>[2x]GALARPCDCDVGGALDPQCDEATGQCRCRPHMIGRRCEQVQPGYFRPFLDHLTWEAEGAHGQVLEVVERLVTNRETPSWTGVGFVRLREGQEVEFLVTSLPRAMDYDLLLRWEPQVPEQWAELELVVQRPGPVSAHSPCGHVLPRDDRIQGMLHPNTRVLVFPRPVCLEPGLSYKLKLKLTGTGGRAHPETPYSGSGILIDSLVLQPHVLMLEMFSGGDAAALERRTTFERYRCHEEGLMPSKTPLSEACVPLLISASSLVYNGALPCQCDPQGSLSSECNPHGGQCRCKPGVVGRRCDACATGYYGFGPAGCQA

Heterotrimeric (αβγ) laminins are a major constituent of all basement membranes. A major function of laminins is to form cell-associated polymers, which provide structural support as well as platforms for signalling. The three short arms of the laminin heterotrimer are composed of long repeats of laminin-type epidermal growth factor-like (LE) domains, capped by laminin N-terminal (LN) domains that mediate the self-interaction of laminins. The LE repeats are interrupted once (β and γ chains) or twice (α chains) by globular domains of unknown function.

The β2 LE5-LF-LE6 structure was solved by the multiple isomorphous replacement method and refined to Rfree = 0.210 at 1.85 Å resolution. The asymmetric unit of the monoclinic crystals contains two structurally very similar copies of β2 LE5-LF-LE6 (r.m.s. deviation of 0.62 Å for 301 Cα atoms). The β2 LE5-LF-LE6 fragment has a surprisingly compact structure with approximate dimensions of 60 Å × 50 Å × 40 Å. The 220 residues inserted between LE5 and LE6 are folded into two distinct regions, a 10-stranded β-sandwich (residues 564–726) and an α-helical region (727–783). The Ca2 + ion is coordinated by the side chains of Glu573 (monodentate), Glu575 (bidentate) and Asp719 (monodentate), as well as the carbonyl oxygen atoms of residues 598, 601 and 719; the resulting coordination geometry is a pentagonal bipyramid. The α-helical region of the LF domain consists of three helices held together by a disulphide bond, Cys752–Cys768, and a substantial hydrophobic core (Val727, Leu730, Met732, Phe733, Phe747, Leu771, Leu772, Ala775, Val779) that is conserved in other LF domains. Helix α3 plays an important role in mediating the apparently stable association of the LF domain with LE5: α3 residues Ser774 and Ser776 interact with loop a of LE5 (residues 528–531), and Gly782 and Val783 interact with loop c of LE5 (residues 547–550). A search for related structures using PDBeFold revealed that the β-sandwich of the LF domain is related to the family 35 carbohydrate binding module (CBM35) structure, despite pairwise sequence identities of just over 10%; the α-helical region of the LF domain has no counterpart in CBM35 or any other protein. An unexpected feature of the laminin β2 LE5-LF-LE6 structure is the relative arrangement of LE5 and LE6, which closely resembles the canonical arrangement of LE domains that are not separated by an inserted domain. Thus, the LF domain is inserted into the short arm of laminin β chains without interrupting the regular array of LE domains.> MLEQMISSSKVGVKINEWYKYIRLFSVPDSEIL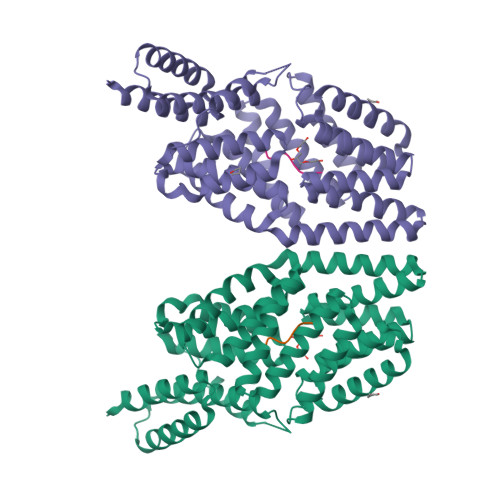KAEVEEEIRHMKEDHDLLLYYSLMCFRHQLMLDYLEPKTLNEERPKISDLLEKIESSQTDLKGILEYYFNFFRGMYEFEQYEYLNAISFYKQAERKLSLVADEIERAEFHYKVAEIYYHMKQTHMSMHHIVQAIDSYKAHENYTVRVIQCSFVIGLNYLDMDYPEKAIPHFKNALDKAREIDMSRLIGSSLYNLGLCSFAEEAYEKASEYFKEGIRVYQDNGYEHSNRILDILLMLTKTTFKMRNHSEGISWCAHGLSLSKNLNDEIMAKMFEFIHALYVDNDNEKLNSILNYLELKSMLSDVEDLASDAAKYYNEKEDHKVAVAYYEKVLYARKQIQRGDCLYET;> SRGHTS Target-based azole resistance in Candida albicans involves overexpression of the ERG11 gene encoding lanosterol 14α-demethylase (LDM), and/or the presence of single or multiple mutations in this enzyme. The azole antifungals inhibit sterol 14α-demethylase (CYP51, SDM), thereby preventing biosynthesis of the essential and fungal specific sterol ergosterol, and resulting in the collateral synthesis of toxic sterols. We have used, as surrogates, structurally aligned mutations in recombinant hexahistidine-tagged full-length Saccharomyces cerevisiae LDM6×His (ScLDM6×His) to elucidate how differential susceptibility to azole drugs is conferred by LDM of the C. albicans Darlington strain. Phenotypes and high-resolution X-ray crystal structures were determined for the surrogate enzymes in complex with representative short-tailed (voriconazole) and long-tailed (itraconazole) triazoles.

Boat-shaped crystals were also obtained using Ni-NTA affinity and SEC purified ScErg11p6×His I471T mutant in complex with either ITC or VCZ. These formed within one week across all experimental conditions tested (43–46% PEG 400 and 0.5 M glycine, pH 9.1–9.6). While we were unable to differentiate the ScLDM6×His wild-type and I471T structures from the mutation at I471, we detected spectral changes consistent with modification of the electronic environment of the heme. Furthermore, consistent with functional modification of the heme, the insertion of I471T into the hydrophobic environment near K151 gave blue shifts to 416 nm in both ScLDM6×His I471T and ScLDM6×His Y140H I471T preparations, as well as lower spectral responses to the binding of VCZ by ScLDM6×His I471T. The presence of the I471T mutation reduced the spectral response due to type II binding of VCZ and ITC, with the major difference observed in the trough region of the difference spectrum. Despite these changes, the type II binding curves showed that both VCZ and ITC bound tightly to the wild-type and I471T mutant enzymes, with each drug giving IC50 values of ~0.6–0.8 µM in the presence of 2 µM enzyme. The appearance of the AO seems more complicated and requires either small (ScLDM6×His Y140F in complex with FLC) or larger (ScLDM6×His or ScLDM6×His I471T in complex with VCZ) changes in conformation of M509, plus a modified conformation of the H317 sidechain in helix I involved in the proton channel. ScLDM6×His in complex with ITC shows that the long tail of ITC occupies the SEC, with M509 adopting a conformation closely matching that found in ScLDM6×His Y140F and ScLDM6×His Y140F I471T complexed with VCZ, but not ScLDM6×His or ScLDM6×His I471T complexed with VCZ. The capture of the water molecule by ScLDM6×His I471T complexed with ITC but not the complex with VCZ may have implications for catalytic efficiency.

> MSATKSIVGEALEYVNIGLSHFLALPLAQRISLIIIIPFIYNIVWQLLYSLRKDRPPLVFYWIPWVGSAVVYGMKPYEFFEECQKKYGDIFSFVLLGRVMTVYLGPKGHEFVFNAKLADVSAEAAYAHLTTPVFGKGVIYDCPNSRLMEQKKFVKGALTKEAFKSYVPLIAEEVYKYFRDSKNFRLNERTTGTIDVMVTQPEMTIFTASRSLLGKEMRAKLDTDFAYLYSDLDKGFTPINFVFPNLPLEHYRKRDHAQKAISGTYMSLIKERRKNNDIQDRDLIDSLMKNSTYKDGVKMTDQEIANLLIGVLMGGQHTSAATSAWILLHLAERPDVQQELYEEQMRVLDGGKKELTYDLLQEMPLLNQTIKETLRMHHPLHSLFRKVMKDMHVPNTSYVIPAGYHVLVSPGYTHLRDEYFPNAHQFNIHRWNNDSASSYSVGEEVDYGFGAISKGVSSPYLPFGGGRHRCTGEHFAYCQLGVLMSIFIRTLKWHYPEGKTVPPPDFTSMVTLPTGPAKIIWEKRNPEQKIGGRHHHHHH>[4x]TRDQNGTWEMESNENFEGYMKALDIDFATRKIAVRLTQTKVIDQDGDNFKTKTTSTFRNYDVDFTVGVEFDEYTKSLDNRHVKALVTWEGDVLVCVQKGEKENRGWKQ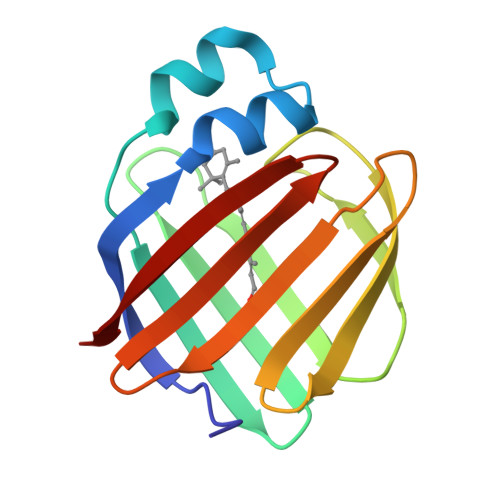WIEGDKLYLELTCGDQVCRQVFKKK> MEGTGVVAVYGNGAITEAKKSPFSVKVGLAQMLRGGVIMDVVNAEQARIAEEAGACAVMALERVPADIRAQGGVARMSDPQMIKEIKQAVTIPVMAAARIGHFVEAQILEAIGIDYIDESEVLTLADEDHHINKHNFRIPFVCGCRNLGEALRRIREGAAMIRTKGEAGTGNIIEAVRHVRSVNGDIRVLRNMDDDEVFTFAKKLAAPYDLVMQTKQLGRLPVVQFAAGG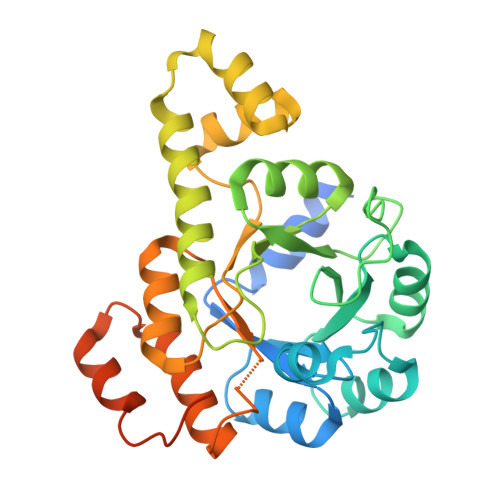VATPADAALMMQLGCDGVFVGSGIFKSGDPARRARAIVQAVTHYSDPEMLVEVSCGLGEAMVGINLNDEKVERFANRSEHHHHHH EmbB and EmbC have mutations known to lead to ethambutol resistance, while a clear effect of the drug on EmbA activity has not been established.

Using single-particle cryogenic electron microscopy (cryo-EM), we determined the structure of EmbB from M. smegmatis expressed in E. coli and reconstituted in lipid-filled nanodiscs to 3.3 Å resolution. Here, EmbB appears as a monomer, consisting of 15 TM helices and two distinct periplasmic carbohydrate binding modules (CBMs). The next 11 TM helices adopt a typical GT-C glycosyltransferase fold, structurally similar to enzymes from various glycosyltransferase families: mycobacterial AftD from GT5315, archaeal ArnT from GT8316, yeast Pmt1-Pmt2 from GT3917, and bacterial PglB from GT6618. EmbB has a single large cavity (volume of ~1120 Å3) at the membrane–periplasm interface that encompasses juxtamembrane (JM) helix 4 and a disordered stretch of around 20 residues between JM4 and TM10. Conservation analyses reveal that this cavity contains highly conserved charged residues (D285, D286, R389, E391), where the residues corresponding to D285 and D286 are required for catalytic activity of corynebacterial EmbB (D297 and D298)19 and mycobacterial EmbC (D293 and D294)20. Based on this structural comparison, the lipidic donor (DPA) is likely to bind in the pocket formed by TM helices 7–9, on the right side of the cavity, with the soluble acceptor substrate binding to the left. We observe two bound lipids in our structure, in a pocket formed by TM helices 2, 5, 6, 7, and 9 on opposite leaflets. A tightly bound phosphatidylglycerol lipid and calcium cation that likely serve a structural purpose were evident in the density map, and their presence and identity were confirmed using native and denaturing mass spectrometry. Focusing only on residues conserved between M. tuberculosis and M. smegmatis, we found that mutations causing resistance all cluster around the putative active site. Notably, these mutations are closer to the putative DPA binding site, suggesting that ethambutol might interfere with recruitment of the arabinose donor, thereby inhibiting enzyme function.

> MSGNMDEAVSGNMDEAVSAGKDVRIARWVATIAGLLGFVLSVSIPLLPVTQTTATLNWPQQGRLDNVTAPLISQAPLELTATVPCSVVRDLPPEGGLVFGTAPAEGRDAALNAMLVNVTETRVDVIVRNVVVASVNRDRVAGPDCQRIEITSNLDGTYADFVGLTQISGEDAGKLQRTGYPDPNLRPAIVGVFTDLTGPAPQGLSVSAEIDTRFTTHPTALKLAAMLLAIVSTVIALLALWRLDRLDGRRMHRLIPTRWRTVTAVDGVVVGGMAIWYVIGANSSDDGYILQMARTAEHAGYMANYFRWFGSPEDPFGWYYNVLALMTKVSDASIWIRLPDLICALICWLLLSREVLPRLGPAVAGSRAAMWAAGLVLLGAWMPFNNGLRPEGQIATGALITYVLIERAVTSGRLTPAALAITTAAFTLGIQPTGLIAVAALLAGGRPILRIVMRRRRLVGTWPLIAPLLAAGTVILAVVFADQTIATVLEATRIRTAIGPSQEWWTENLRYYYLILPTTDGAISRRVAFVFTAMCLFPSLFMMLRRKHIAGVARGPAWRLMGIIFATMFFLMFTPTKWIHHFGLFAAVGGAMAALATVLVSPTVLRSARNRMAFLSLVLFVLAFCFASTNGWWYVSNFGAPFNNSVPKVGGVQISAIFFALSAIAALWAFWLHLTRRTESRVVDRLTAAPIPVAAGFMVVVMMASMAIGVVRQYPTYSNGWANIRAFAGGCGLADDVLVEPDSNAGFLTPLPGAYGPLGPLGGEDPQGFSPDGVPDRIIAEAIRLNNPQPGTDYDWNRPIKLDEPGINGSTVPLPYGLDPKRVPVAGTYSTEAQQESRLSSAWYELPARDETERAAHPLVVITAAGTITGESVANGLTTGQTVDLEYATRGPDGTLVPAGRVTPYDVGPTPSWRNLRYPRSEIPDDAVAVRVVAEDLSLSQGDWIAVTPPRVPELQSVQEYVGSDQPVLMDWAVGLAFPCQQPMLHANGVTEVPKFRISPDYYAKLQSTDTWQDGINGGLLGITDLLLRASVMSTYLSQDWGQDWGSLRKFDTVVEATPAELDFGSQTHSGLYSPGPLRIRPAENLYFQGWSHPQFEK>MATNNNQIGENKEQTIFDHKGNVIKTEDREIQIISKFEEPLIVVLGNVLSDEECDELIELSKSKLARSKVGSSRDVNDIRTSSGAFLDDNELTAKIEKRISSIMNVPASHGEGLHILNYEVDQQYKAHYDYFAEH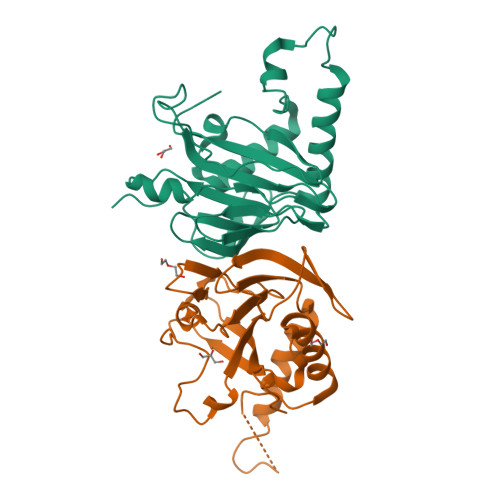SRSAANNRISTLVMYLNDVEEGGETFFPKLNLSVHPRKGMAVYFEYFYQDQSLNELTLHGGAPVTKGEKWIATQWVRRGTYK[2x]> MKRHLILLFVGVSLPFLLAAQQKNSVSITKRVLRIPEVTVVGKRPMKDIGVQRTRFDSIAMKENIALSMADVLTFNSSVFVKNYGRATLSTVAFRGTSPSHTQVTWNGMRINNPMLGMTDFSTIPSYFIDDASLLHGTSSVNETGGGLGGLVRLSTSPANHEGFGLQYVQGVGSFSTFDEFLRLTYGDKHWQSSTRVVYSSSPNDYKYRNRDKKENIYDEDKNIIGSYYPTERNRSGAYKDLHVLQEIYYNTGEGDKFGLNAWYINSNRELAMLSTDYGNDMDFENRQREQTFRGVLSWDRVREKWKVGVKGGYIHTWMAYDYKRDKGNGEMASMTRSRSKINTFYGSADGDYAPSEKWLFTAGVSVHQHLVESADKNIISQEGNKAVVGYDKGRVEFSGSVSAKWRPVDRFAASLVLREDMFGTEWAPVIPAFFIDGVLSKKGNIVAKASISRNYRFPTLNDLYFLPGGNPDLKSEHGFTYDVGLSFSVGKENVYALSGGINWFDSHIDDWIIWLPTTKGFFSPRNLKKVHAYGAETNAHLDIMLGKDWKLDMNGTFSWTPSINESEPMSPADQSVGKQLPYVPEFSATVTGRLSWRTWSLLYKWCYYSQRYTMSSNDYTLTGYLPPYFMNNVTL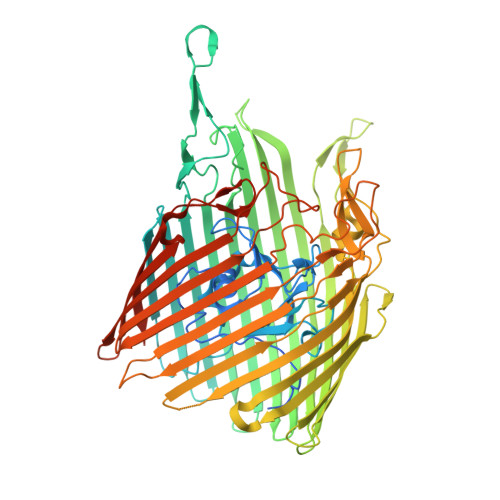EKQLSFRWADLSLKGSINNLFDEEYLSVLSRPMPGINFEIFIGITPKFGKNKNSKRHHHHHH>[2x]DDHSELLVNTKSGKVMGTRVPVLSSHISAFLGIPFAEPPVGNMRFRRPEPKKPWSGVWNASTYPNNCQQYVDEQFPGFSGSEMWNPNREMSEDCLYLNIWVPSPRPKSTTVMVWIYGGGFYSGSSTLDVYNGKYLAYTEEVVLVSLSYRVGAFGFLALHGSQE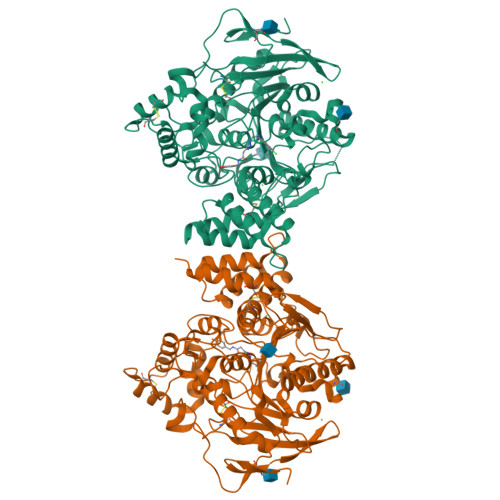APGNVGLLDQRMALQWVHDNIQFFGGDPKTVTIFGESAGGASVGMHILSPGSRDLFRRAILQSGSPNCPWASVSVAEGRRRAVELGRNLNCNLNSDEELIHCLREKKPQELIDVEWNVLPFDSIFRFSFVPVIDGEFFPTSLESMLNSGNFKKTQILLGVNKDEGSFFLLYGAPGFSKDSESKISREDFMSGVKLSVPHANDLGLDAVTLQYTDWMDDNNGIKNRDGLDDIVGDHNVICPLMHFVNKYTKFGNGTYLYFFNHRASNLVWPEWMGVIHGYEIEFVFGLPLVKELNYTAEEEALSRRIMHYWATFAKTGNPNEPHSQESKWPLFTTKEQKFIDLNTEPMKVHQRLRVQMCVFWNQFLPKLLNATACDGELSSSGTSSSKGIIFYVLFSILYLIF(R)-ketamine 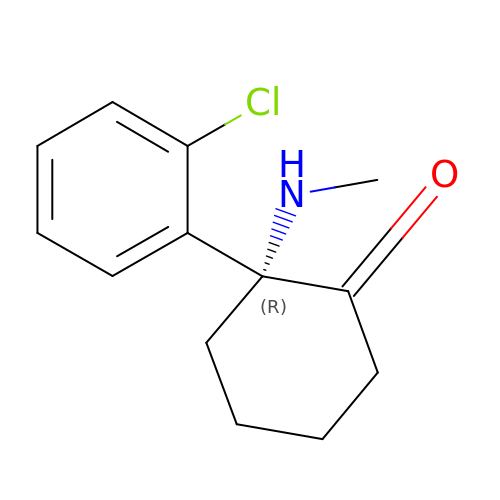| C13 H16 Cl N O | YQEZLKZALYSWHR-CYBMUJFWSA-N> CDIHVLWEWKCFEDL;>[2x]EVVKFMDVYQRSYCHPIETLVDIFQEYPDEIEYIFKPS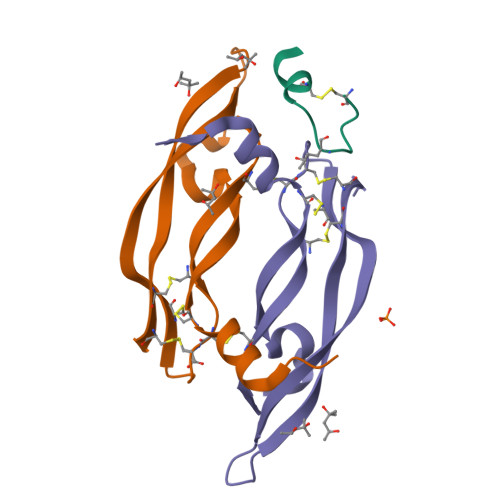CVPLMRCGGCCNDEGLECVPTEESNITMQIMRIKPHQGQHIGEMSFLQHNKCECRPK> FEDRDPTQFEERHLKFLQQLGKGNFGSVEM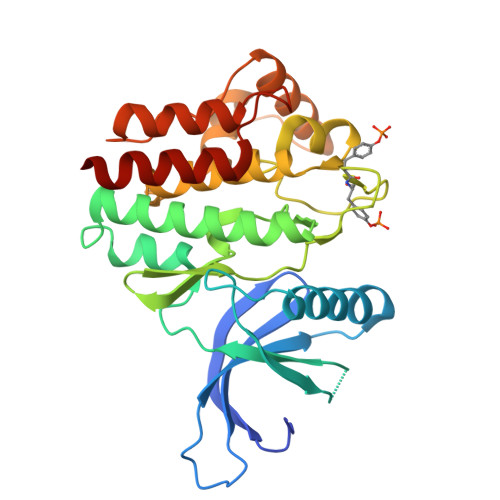CRYDPLQDNTGEVVAVKKLQHSTEEHLRDFEREIEILKSLQHDNIVKYKGVCYSAGRRNLRLIMEYLPYGSLRDYLQKHKERIDHKKLLQYTSQICKGMEYLGTKRYIHRDLATRNILVENENRVKIGDFGLTKVLPQDKEYYKVKEPGESPIFWYAPESLTESKFSVASDVWSFGVVLYELFTYIEKSKSPPVEFMRMIGNDKQGQMIVFHLIELLKSNGRLPRPEGCPDEIYVIMTECWNNNVSQRPSFRDLSLRVDQIRDSIAA>MSKIKNPILTGFHPGPSICRVGDDYYIAVSTFEWFPGVRIYHSKDLKNWRLVARPLNRLSQLNMIGNPDSGGVWAPHLSYSDGKFWLIYTDVKVVEGQWKDGHNYLVTCDTIDGAWSDPIYLNSSGFDPSLFHDEDGRKYLVNMYWDHRVDHHPFYGIVLQEYSVEQKKLVGEPKIIFKGTDLRITEGPHLYKINGYYYLLTAEGGTRYNHAATIARSTSLYGPYEVHPDNPLLTSWPYPRNPLQKAGH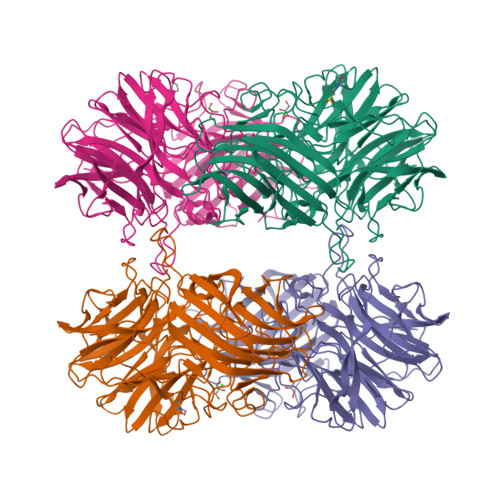ASIVHTHTDEWFLVHLTGRPLPREGQPLLEHRGYCPLGRETAIQRLEWKDGWPYVVGGNGPSLEIDGPSVEEVSWEKDYDEKDDFDGDTLNHHFQTLRIPLGEDIATLKARPGHLRLYGRESLTSRFTQAFVARRWQHFHFVAETKVSFRPTTFQQSAGLVNYYNTQNWTTLQITWHEEKGRILELMTCDHLVVDQPLRGREIVVPDDIEYVYLRVTVQATTYKYSYSFDGMNWIDLPVTFESYKLSDDYIKSRAAFTGAFVGMHCRDGSGQNNYADFDYFLYKEL[4x]>MSRVTVLQSQLPAYNRLKTPYESELIATVKKLTTPGKGLLAADESIGSCTKRFQPIGLSNTEEHRRQYRALMLEAEGFEQYISGVILHDETVGQKASNGQTFPEYLTARGVVPGIKTDMGLCPLLEGAEGEQMTEGLDGYVKRASAYYKKG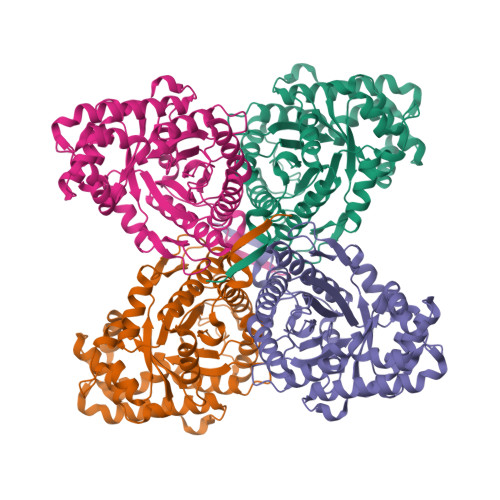CRFCKWRNVYKIQNGTVSESAVRFNAETLARYAILSQMSGLVPIVEPEVMIDGKHDIDTCQRVSEHVWREVVAALQRHGVIWEGCLLKPNMVVPGAESGKTAAPEQVAHYTVMTLARTMPAMLPGVMFLSGGLSEVQASEYLNAINNSPLPRPYFLSFSYARALQSSALKAWGGKESGLAAGRRAFLHRARMNSMAQLGKYKRSDDDASSSSLYVKGNT[4x]> GIQSYCTPPYSVLQDPPQPVVWRRYMLYDCVFDFTVVVDSLPTHQLQCYGVSPRRLAS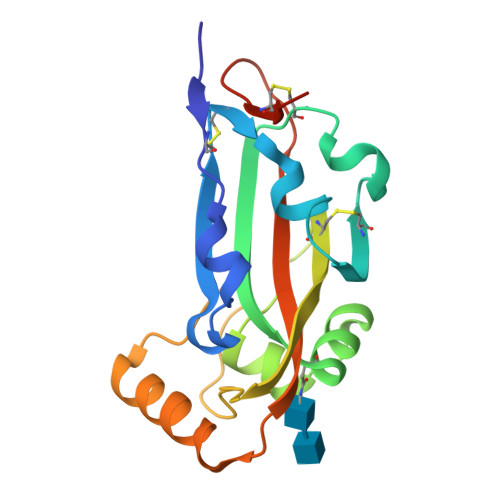MCYGSVTLDVMRINETHLNNLFNRVPDTFSLYNYALPDNFYGCLHAFYLNSTAPYAVANRFPIKPGGRQSNSAFIDTVINAAHYSPFSYVYGLAVITLKPAAGSKLVCPVANHHHHHH>[2x]MVKKPPKSYDEYKQVDVGKDGMVATAHPLASEIGADVLKKGGNAIDAAVAIQFALNVTEPMMSGIGGGGFMMVYDGKTKDTTIIDSRERAPAGATPDMFLDENGKAIPFSERVTKGTAVGVPGTLKGLEEALDKWGTRSMKQLITPSIKLAEKGFPIDSVLAEAISDYQEKLSRTAAKDVFLPNGEPLKEGDTLIQKDLAKTFKLIRSKGTDAFYKGKFAKTLSDTVQDFGGSMTEKDLENYDITIDEPIWGDYQGYQIATTP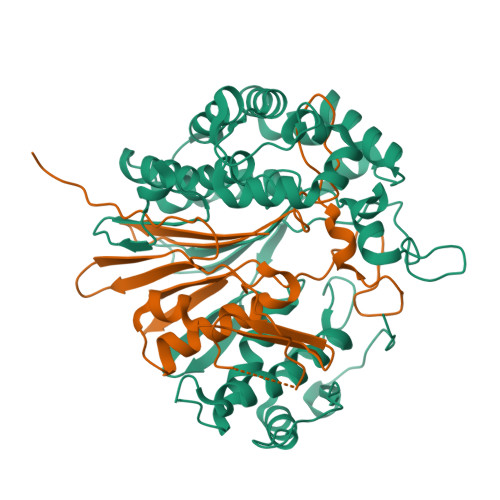PPSSGGIFLLQMPKILDHFNLSQYDVRSWEKYQLLAETMHLSYADRASYAGDPEFVNVPLKGLLHPDYIKERQQLINLDQVNKKPKAGDPWKYQEGSANYKQVEQPKDKVEGQ;>TTHFTVADRWGNVVSYTTTIEQLFGTGIMVPDYGVILNNELTDFDAIPGGANEVQPNKRPLSSMTPTILFKDDKPVLTVGSPGGATIISSVLQTILYHIEYGMELKAAVEEPRIYTNSMSSYRYEDGVPKDVLSKLNGMGHKFGTSPVDIGNVQSISIDHENGTFKGVADSSRNGAAIGINLKRKLEHHHHHH[2x]>[2x]GPH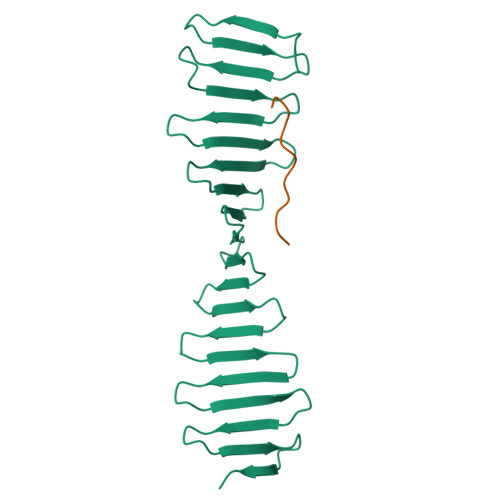MEEIMQSDSKIEKMLPDGGRLVVFPNGTRKELSADGQTVKVMFFNGDVKHTMPDQRVIYYYAEAQTTHITYPDGMEVLQFPNNQTEKHFPDGRKEITFPDQTVKTLHPDGREESVLTDGTIIQLNPDGSKVIQFNTGQREIHTADFKRREYPDGTVKTVYSDGRQETQYPTGRVRLKDPQGKVIMDTKA;>GSGVEDEDLSPRPSPNPHPVSQENLYFQ[2x]>[12x]MNIMDFNVKKLAADAGTFLSRAVQFTEEKLGQAEKTELDAHLENLLSKAECTKIWTEKIMKQTEVLLQPNPNARIEEFVYEKLDRKAPSRINNPELLGQYMIDAGTEFGPGTAYGNALIKCGETQKRIGTADRELIQTSALNFLTPLRNFIEGDYKTIAKERKLLQNKRLDLDAAKTRLKKAKAAETRNSSEQELRITQSEFDRQAEITR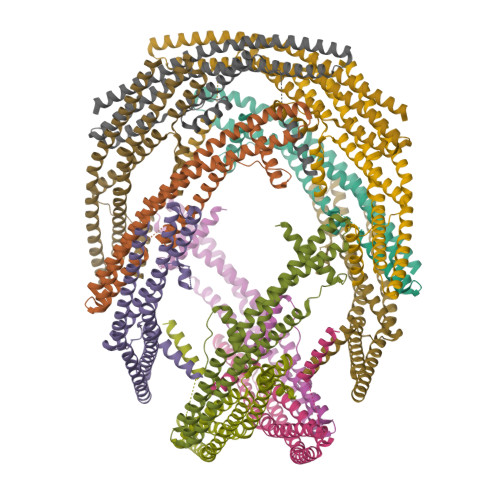LLLEGISSTHAHHLRCLNDFVEAQMTYYAQCYQYMLDLQKQLGSFPSNYLSNNNQTSVTPVPSVLPNAIGSSAMASTSGLVITSPSNLSDLKECSGSRKARVLYDYDAANSTELSLLADEVITVFSVVGMDSDWLMGERGNQKGKVPITYLELLN>VPRGGHMFMRVEKIMNSNFKTVNWNTTVFDAVKIMNENHLYGLVVKDDNGNDVGLLSERSIIKRFIPRNKKPDEVPIRLVMRKPIPKVKSDYDVKDVAAYLSENGLERCAVVDDPGRVVGIVTLTDLSRYLSRASITDILLSHRTKDYQHLCPKCGVGVLEPVYNEKGEIKV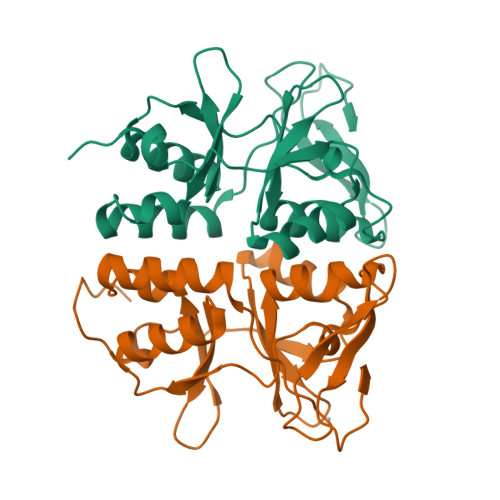FRCSNPACDYEE[2x]>[2x]MAEDKSKRDSIEMSMKGCQT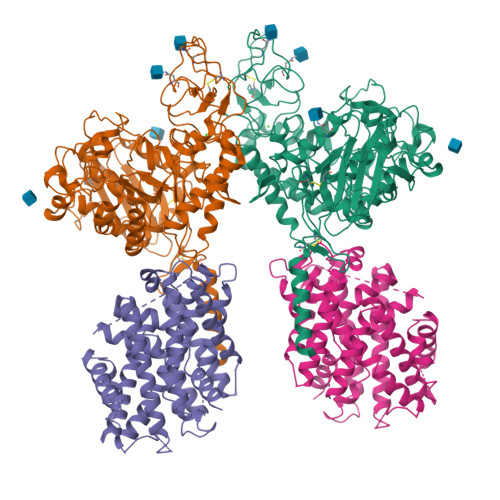NNGFVHNEDILEQTPDPGSSTDNLKHSTRGILGSQEPDFKGVQPYAGMPKEVLFQFSGQARYRIPREILFWLTVASVLVLIAATIAIIALSPKCLDWWQEGPMYQIYPRSFKDSNKDGNGDLKGIQDKLDYITALNIKTVWITSFYKSSLKDFRYGVEDFREVDPIFGTMEDFENLVAAIHDKGLKLIIDFIPNHTSDKHIWFQLSRTRTGKYTDYYIWHDCTHENGKTIPPNNWLSVYGNSSWHFDEVRNQCYFHQFMKEQPDLNFRNPDVQEEIKEILRFWLTKGVDGFSLDAVKFLLEAKHLRDEIQVNKTQIPDTVTQYSELYHDFTTTQVGMHDIVRSFRQTMDQYSTEPGRYRFMGTEAYAESIDRTVMYYGLPFIQEADFPFNNYLSMLDTVSGNSVYEVITSWMENMPEGKWPNWMIGGPDSSRLTSRLGNQYVNVMNMLLFTLPGTPITYYGEEIGMGNIVAANLNESYDINTLRSKSPMQWDNSSNAGFSEASNTWLPTNSDYHTVNVDVQKTQPRSALKLYQDLSLLHANELLLNRGWFCHLRNDSHYVVYTRELDGIDRIFIVVLNFGESTLLNLHNMISGLPAKMRIRLSTNSADKGSKVDTSGIFLDKGEGLIFEHNTKNLLHRQTAFRDRCFVSNRACYSSVLNILYTSC;>MGDTGLRKRREDEKSIQSQEPKTTSLQKELGLISGISIIVGTIIGSGIFVSPKSVLSNTEAVGPCLIIWAACGVLATLGALCFAELGTMITKSGGEYPYLMEAYGPIPAYLFSWASLIVIKPTSFAIICLSFSEYVCAPFYVGCKPPQIVVKCLAAAAILFISTVNSLSVRLGSYVQNIFTAAKLVIVAIIIISGLVLLAQGNTKNFDNSFEGAQLSVGAISLAFYNGLWAYDGWNQLNYITEELRNPYRNLPLAIIIGIPLVTACYILMNVSYFTVMTATELLQSQAVAVTFGDRVLYPASWIVPLFVAFSTIGAANGTCFTAGRLIYVAGREGHMLKVLSYISVRRLTPAPAIIFYGIIATIYIIPGDINSLVNYFSFAAWLFYGLTILGLIVMRFTRKELERPIKVPVVIPVLMTLISVFLVLAPIISKPTWEYLYCVLFILSGLLFYFLFVHYKFGWAQKISKPITMHLQMLMEVVPPEEDPE[2x]>[4x]MSAEGYQYRALYDYKKEREEDIDLHLGDILTVNK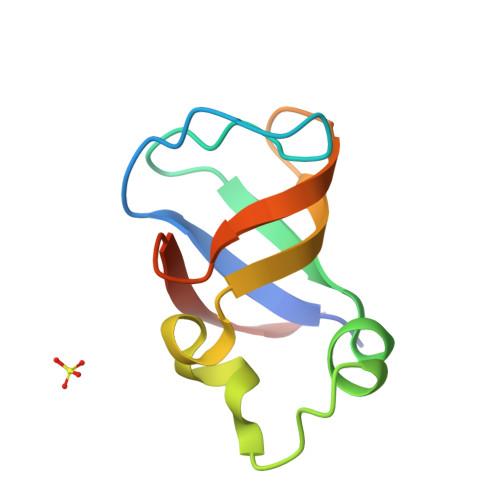GSLVALGFSDGQEARPEEIGWLNGYNETTGERGDFPGTYVEYIGRKKIS2-(2,4-DICHLORO-PHENOXY)-N-(2-MERCAPTO-ETHYL)-ACETAMIDE 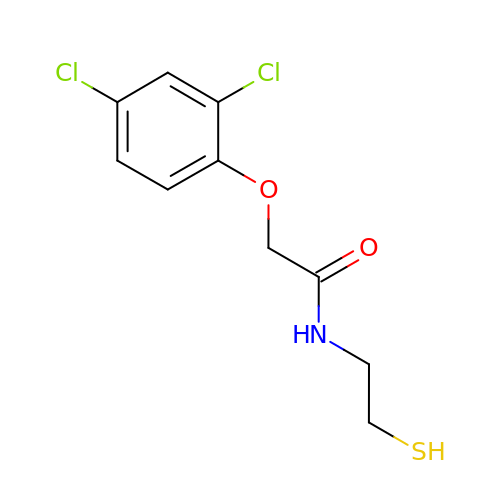| C10 H11 Cl2 N O2 S | ZKLFUOFLXGWIIY-UHFFFAOYSA-N> GSTGSPPGPPTSIHVEEITDTTATLSWRPGPDNHSPITAYTIQARTPFSLGWQAVSTVPEVVGGSHLTATVIELNPWVEYEFRVLASNAVGTGEPSKPSKKARTKDTVPKVTPANVSGGGGSRSELVITWEPVPEELQNGAGFGYVVAFRPFGSTGWMQAAVPSPEASKYVFKNETILPFSPFQVKVGAYNNKGEGPFGPVITIYSAEEEPGRAPSRLRAKSLSASDVEVSWKALPWSTSKKRVLGYELRYWEKNEKEDASSVLRTVGNRTLAIIQGLKGSSTYYITVRAYNTAGTGPPSPVVNITTKK

Contactins (CNTNs) are neural cell adhesion molecules that encode axon-target specificity during the patterning of the vertebrate visual and olfactory systems. Because CNTNs are tethered to the plasma membrane by a glycosylphosphatidylinositol anchor, they lack an intracellular region to communicate across the membrane. Instead, they form coreceptor complexes with distinct transmembrane proteins to transmit signals inside the cell. Finally, structural analyses of five CNTN–amyloid pairs indicate that these proteins interact through a conserved interface involving the second fibronectin type III repeat of CNTNs and the copper-binding domain of amyloid proteins.

Introducing the T751A and V752A mutations in chicken CNTN4 reduced its affinity for APP by fourfold, so we found it intriguing that these changes occur naturally in zebrafish CNTN4. We thus decided to gain structural insights into the zebrafish complexes to determine the extent to which details of interactions differed when compared with chicken CNTN4–APP. Finally, complex formation does not involve any substantial structural change in CNTN4, since the structure of the unbound FN2 domain in CNTN4 matches those of amyloid-bound CNTN4 closely.>[4x]MNLLSDKNVAIIGGGPVGLTMAKLLQQNGIDVSVYERDNDREARIFGGTLDLHKGSGQEAMKKAGLLQ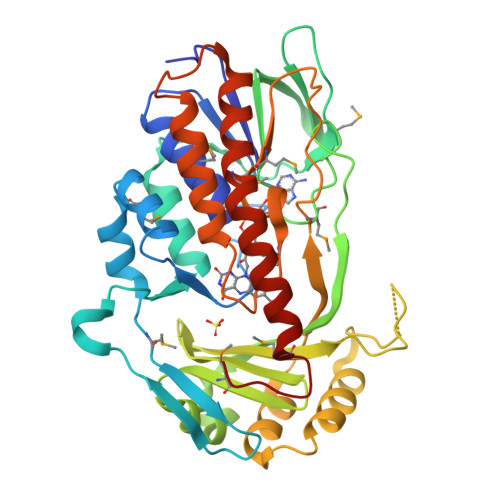TYYDLALPMGVNIADKKGNILSTKNVKPENRFDNPEINRNDLRAILLNSLENDTVIWDRKLVMLEPGKKKWTLTFENKPSETADLVILANGGMSKVRKFVTDTEVEETGTFNIQADIHQPEINCPGFFQLCNGNRLMASHQGNLLFANPNNNGALHFGISFKTPDEWKNQTQVDFQNRNSVVDFLLKKFSDWDERYKELIHTTLSFVGLATRIFPLEKPWKSKRPLPITMIGDAAHLMPPFAGQGVNSGLVDALILSDNLADGKFNSIEEAVKNYEQQMFIYGKEAQEESTQNEIEMFKPDFTFQQLLNV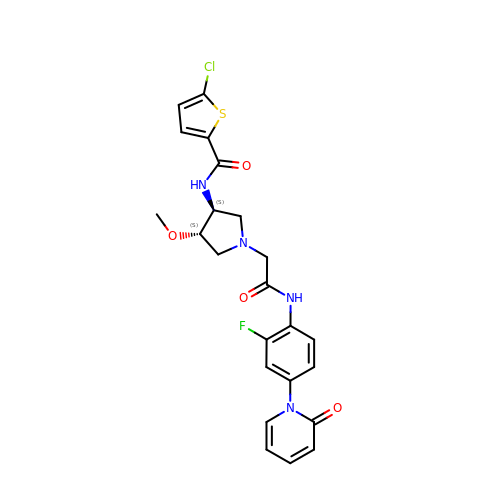5-chloro-N-[(3S,4S)-1-(2-{[2-fluoro-4-(2-oxopyridin-1(2H)-yl)phenyl]amino}-2-oxoethyl)-4-methoxypyrrolidin-3-yl]thiophene-2-carboxamide | C23 H22 Cl F N4 O4 S | BOCLXHFYRGMFSC-ROUUACIJSA-N(2R)-3-[(R)-[(1R)-1-aminoethyl](hydroxy)phosphoryl]-2-methylpropanoic acid | C6 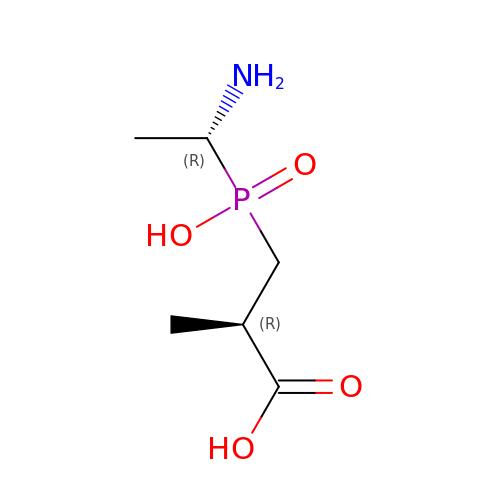H14 N O4 P | XXVGIEKADYFHOF-CRCLSJGQSA-N> HHHHHHSGLVPRGS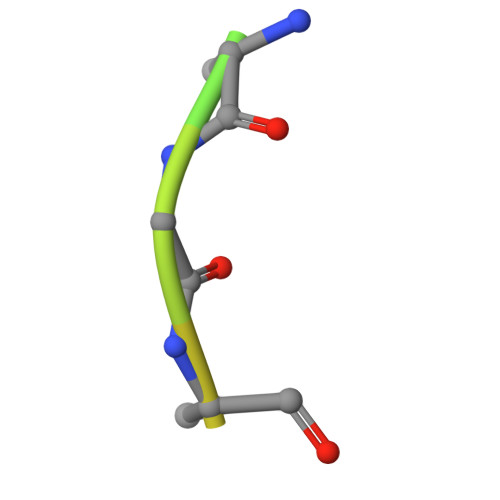HM> MVLLGDVNGDGT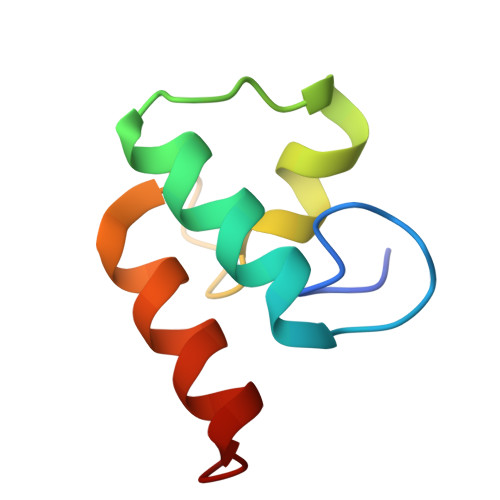INSTDLTMLKRSVLRAITLTDDAKARADVDKNGSINAADVLLLSRYLLRVI Typically, TCSs consist of an histidine kinase (HK) that senses specific external stimuli, and a response regulator (RR) that mediates the cellular response through differential expression of target genes. OmpR/EnvZ is a well-studied TCS in Enterobacteriaceae, where OmpR is the RR and EnvZ is the HK sensor. We demonstrated that OmpR is a key regulator of A. baumannii virulence using different infection models and diverse clinical strains. Overall, the chromosomal mutants impaired for OmpR phosphorylation (D71A) or for DNA binding (R198L) were attenuated similarly to the ΔompR mutant, indicating that both OmpR characteristics are required for A. baumannii virulence.

To enable the discovery of a small molecule inhibitor of OmpR, we solved the crystal structure of OmpRABA DNA binding domain (DBD) spanning the C-terminal residues 148 to 254 at a resolution of 2.2 Å. The analysis of the crystal structure showed that OmpRABA DBD consists of a three-stranded antiparallel β-sheet (β1, V153-F156; β2, W159-D162; β3, R166-T169) followed by three α-helices (α1, T179-E190; α2, R198-R206; α3, R215-I228) and ending with a β-hairpin (β4, I238-V241; β5, V244-F248). The arrangement of the β-sheets and α-helices represents the winged helix-turn-helix (wHTH) fold characteristic of DNA-binding proteins of the OmpR superfamily. The sequence identity between OmpRABA DBD and OmpRECO DBD is 69% and all the amino acid residues of OmpRECO that are involved in the DNA binding were conserved in OmpRABA. These observations suggest a very similar DNA-binding mode for both proteins, which is in line with OmpRABA binding to OmpRECO cognate binding site. The most likely interaction site (hotspot 1) in all structures is around conserved residues T240VWG(V/L)244 in OmpRABA DBD. Residue D218 in chain A may serve as an anchor point. Hotspot 2 in OmpRABA-DBD chain D contains residues S222, R223 and R226 (S206, R207 and R210 in OmpRECO DBD). The “backside” of OmpRABA DBD chain C features a third potential ligand binding pocket flanked by residues K186 (potential anchor residue), L204 and T178/T179. We used our developed D-ELISA to evaluate the inhibitory effect of the virtual hits on OmpRABA DNA binding. We only observed a dose-dependent inhibition of OmpRABA DNA binding for the compound VSIS_039 (STL300125, Vitas-M Chemical Limited), which was identified to bind to the hotspot 2 druggable pocket of OmpR (Figure 6(a,b)).

>MSQQVEVVSFGPWSLDLSTRTLTREGQIVTLTTGEFAVLKALVQHPREPLTRDKLMNLARGREWGAMERSIDVQVSRLRRLIEDNPARARYIQTVWGVGYVFVPDGAEHHHHHH[4x]>MHHHHHHNNDNNTILGFDVNLICDFFLNTERQGPGSPEVTLKALSFIDNLTNKSLIADLGCGTGGQTMILAQHVPGKITGIDFFPGFIERFNKNAEKLNLQNRVKGIVGSMDDLSFEKDSLDLIWSEGAIYNIGFERGLKEWRNYLKPGGYLAVSESVWFTDQRPAEIHDFWMSAYTEIDTVPNKVAQIQKAGYIPVATFILPENCWIEHYFAPQAKAEEIFRRKHAGSRIVEELITSNHHEAELYSKYKAYYGYAFFICKKGFSLRR[2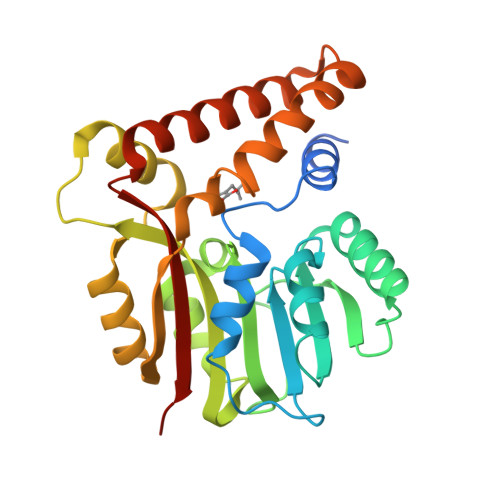x]>KVPRGSHMLNVGATAPDFTLRDQNQQLVTLR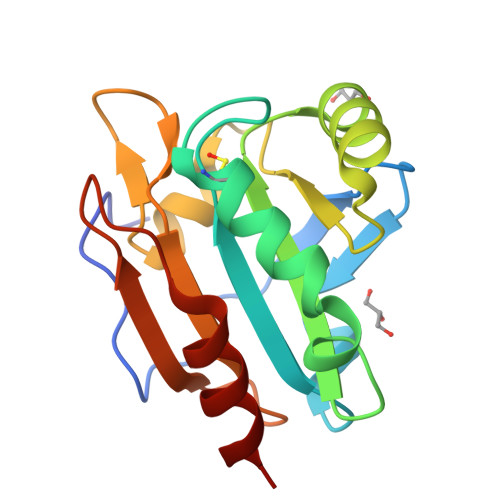GYRGAKNVLLVFFPLAFTGICQGELDQLRDHLPEFENDDSAALAISVGPPPTHKIWATQSGFTFPLLSDFWPHGAVSQAYGVFNEQAGIANRGTFVVDRSGIIRFAEMKQPGEVRDQRLWTDALAALT[2x]> GGCUUCAACA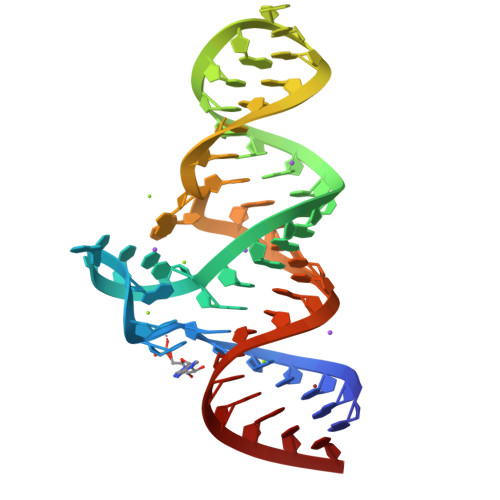ACCCCGUAGGUUGGGCCGAAAGGCAGCGAAUCUACUGGAGCC>MTGGMKPPARKPRILNSDGSSNITRLGLEKRGWLDDHYHDLLTVSWPVFITLITGLYLVTNALFALAYLAVGDVIENARPGSFTDAFFFSVQTMATIGYGKLIPIGPLANTLVTLEALVGMLGLAVAACLIYARCTRPTAGVLFSSRMVISDFEGKPTLMMRLANLRIEQIIEADVHLVLVRSEISQEGMVFRRFHDLTLTRSRSPIFSLSWTVMHPIDHHSPIYGETDETLRNSHSEFLVLFTGHHEAFAQNVHARHAYSSDEIIWGGHFVDV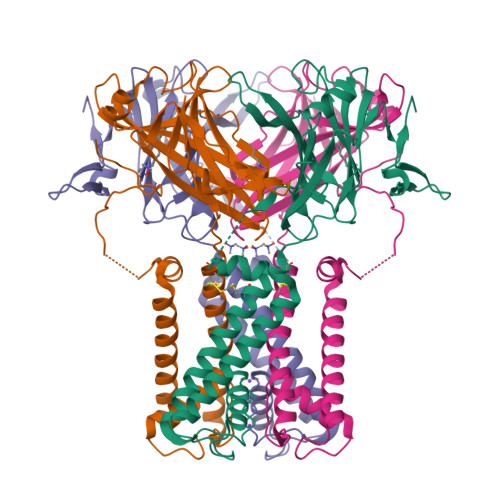FTTLPDGRRALDLGKFHEIAQHHHHHH[2x]>[8x]MAGKAHRLSAEERDQLLPNLRAVGWNE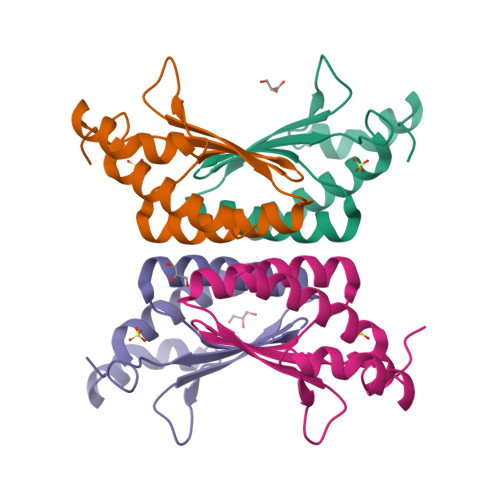LEGRDAIFKQFHFKDFNRAFGFMSRVALQAEKLDHHPEWFNVYNKVHITLSTHECAGLSERDINLASFIEQVAVSMT For more than 25 years, the mainstay of treatment for Schistosoma mansoni infections in Brazil was the drug oxamniquine (OXA, (RS)-1,2,3,4-tetrahydro-2- isopropylaminomethyl-7-nitro-6-quinolylmethanol). The mode of action of OXA was recently elucidated. The resulting sulfate ester of OXA is an unstable species that spontaneously decays to form a reactive electrophilic product capable of alkylating DNA, proteins and other macromolecules. The ensuing disruption of synthetic and metabolic cellular functions eventually leads to parasite death.

OXA possesses one asymmetric carbon atom and its two enantiomers are both present in the marketed drug. Previous studies have succeeded in separating the enantiomers, but have not provided information about their absolute configurations or relative antischistosomal properties. The question of which or if both enantiomers are active, and which or if both can occupy the binding pocket of SmSULT is addressed in this report.

> GAMIESSTTIQVISAGLPRTGTKSLKNALEIIYHKPCYHMFEIIFNKQSDIIKWQNLIHDSHMITTPPPLTTKTIAIYDKLKELLDGYIATTDLPTCGFYKDLMNIYPNAKVLLTIRDKYDWLHSLRKVVLPKSNDPWKLKIEEGDKVLGLNSDFYKLTEDSLKFAFQKDDLNFDDDQVLLECYDEYNRLVQETVPSDRLLVLRLGDGWEPLCKFLNVEIPNGIDYPCVNSHHQMTQLTEQLIKYKSLDAIIHMFPDLI> MIRAVFFDSLGTLISVEGAAKSHLKIMEEVLGDYPLNPKTLLDEYEKLAREAFSNYAGKPYRPLRDILEEVMRKLAEKYGFKYPENLWEIS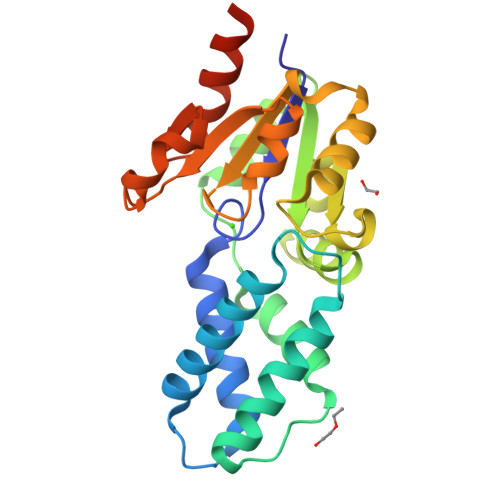LRMSQRYGELYPEVVEVLKSLKGKYHVGMITNRDTEPATAFLDALGIKDLFDSITTSEEAGFFKPHPRIFELALKKAGVKGEKAVYVGDNPVKDAGGSKNLGMTSILLDRKGEKREFWDKADFIVSDLREVIKIVDELNGQGSLEHHHHHH> GSDFSFGPWKLTASKTHIMKSADVEKLADELHMPSLPEMMFGDNVLRIQHGSGFGIEFNATDALRCVNNYQGMLKVACAEEWQEVIKPYDWTYTTDYKGTLLGESLKLKVVPTTDHIDTEKLKAREQIKFFEEVLLFEDELHDHGVSSLSVKIRVMPSSFFLLLRFFLRIDGVLIRMNDTRLYHEADKTYMLREYTSRESKIANLMHV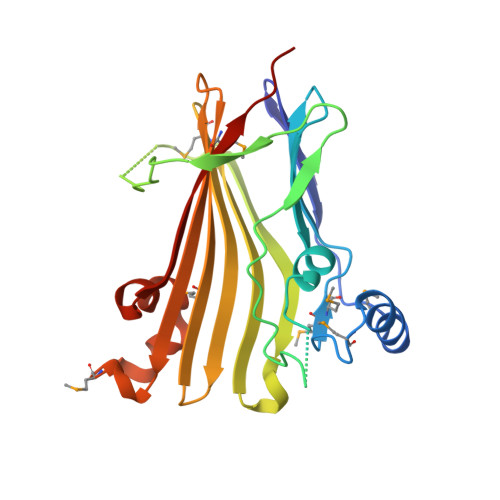PPSLFTEPNEISQYLPIKEAVCEKLVFPERID> DVVVQAPTQVPGFLGDSVTLPCYLQVPNMEVTHVSQLTWARHGESGSMAVFHQTQGPSYSESKRLEFVAARLGAELRNASLRMFGLRVEDEGNYTCLFVTFPQGSR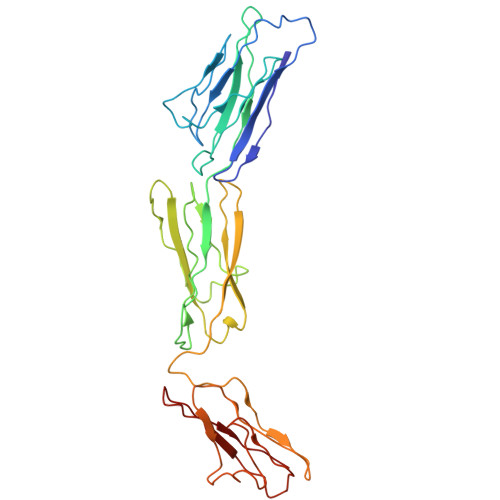SVDIWLRVLAKPQNTAEVQKVQLTGEPVPMARCVSTGGRPPAQITWHSDLGGMPNTSQVPGFLSGTVTVTSLWILVPSSQVDGKNVTCKVEHESFEKPQLLTVNLTVYYPPEVSISGYDNNWYLGQNEATLTCDARSNPEPTGYNWSTTMGPLPPFAVAQGAQLLIRPVDKPINTTLICNVTNALGARQAELTVQV> ETVTPKRM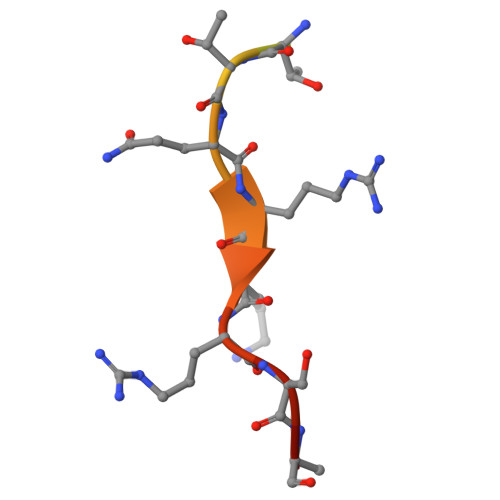RTTQRKRSAT> MAAFVSGGCGVGGQRRAWPAKGAAVARTHACPTTMVVLPVARAGLAATAKKNQYMGTSVAPEIVLTDKGSDMSRKVKTEDKK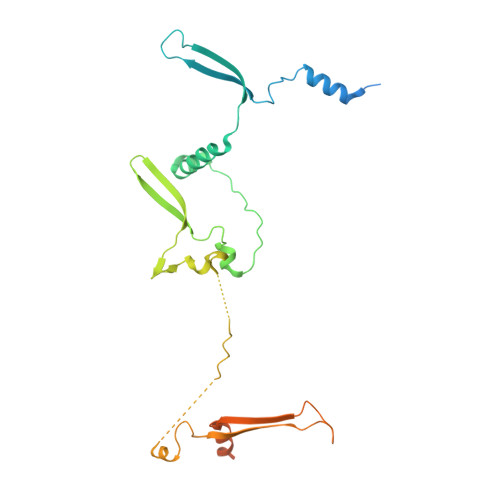VAADQAAAMGILANMSLYASLNPVKRMTYKAKEQAPAYVKKTGNPVEDFYPSSWRNMAPVISLSANRVAVAFEKIDAASNGVKANSNNKPFWKSGATTKNYVAPEAPAQSEPETLDDAAYQRYFPARIRNKAPAMEFRRPSFANTEDPSAYFMLQKETVPLRMALAEKLLTKLGRKGDGSEAEEEKVKPQKKAAKKDAKDDAKDDE>MPSETPQAEVGPTGCPHRSGPHSAKGSLEKGSPEDKEAKEPLWIRPDALSRCTWQLGRPASESPHHHTAPAKSPKILPDILKKIGDTPMVRINKIGKKFGLKCELLAKCEFFNAGGSVKDRISLRMIEDAERDGTLKPGDTIIEPTSGNTGIGLALAAAVRGYRCIIVMPEKMSSEKVDVLRALGAEIVRTPTNARFDSPESHVGVAWRLKNEIPNSHILDQYRNASNPLAHYDTTADEILQQCDGKLDMLVASVGTGGTITGIARKLKEKC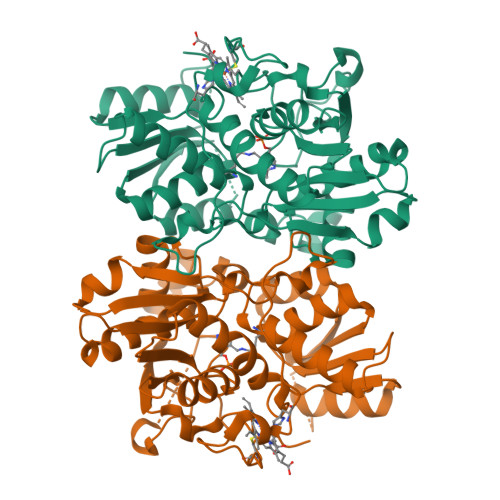PGCRIIGVDPEGSILAEPEELNQTEQTTYEVEGIGYDFIPTVLDRTVVDKWFKSNDEEAFTFARMLIAQEGLLCGGSAGSTVAVAVKAAQELQEGQRCVVILPDSVRNYMTKFLSDRWMLQKGFLKEEDLTEKKPW[6x]2-O-[(R)-hydroxy(propan-2-yloxy)phosphoryl]-alpha-L-arabinopyranose 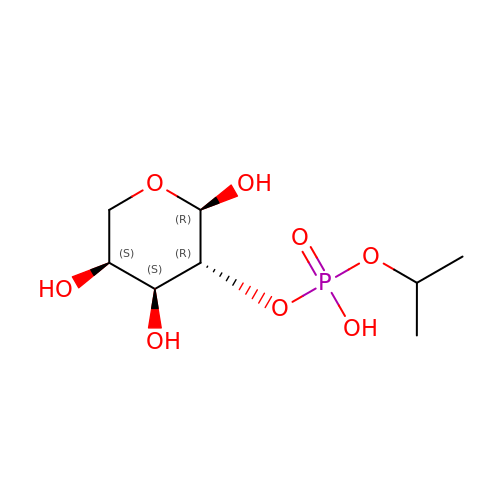| C8 H17 O8 P | PYOXTDKMFCLRNS-RULNZFCNSA-N SV40 T-ag is a 708–amino acid protein containing at least three independent functional domains: an N-terminal J domain (amino acids 1–130), a central origin binding domain (obd) (amino acids 131–260), and a C-terminal helicase domain (amino acids 266–625). In the case of SV40, a single virally encoded initiator, large T-antigen (T-ag), can bind the SV40 origin, assemble as a set of two hexameric rings, and cause local distortions (ie, melting) of the DNA. The T-ag obd recognizes the GAGGC-containing duplex DNA at the origin and also binds double-stranded DNA (dsDNA) and ssDNA in a non–sequence-specific manner. In this paper we describe two crystal structures of the SV40 large T-ag obd: one in complex with duplex DNA and one as a dimer in the absence of DNA.

The crystal structure of the SV40 T-ag obd (amino acids 131–260) with duplex DNA containing two high-affinity binding sites, P1 and P3, was refined to 2.4-Å resolution. Pentanucleotide binding site P2 has been altered to abrogate site-specific binding. The asymmetric unit contains two T-ag obd subunits and a DNA duplex 21 nucleotides long. The two T-ag obds are oriented head-to-head on approximately the same face of the DNA and make almost identical DNA interactions with their respective GAGGC sequences. The DNA positions the obds such that the residues within the B3 loop (amino acids 213–220) are facing each other in an antiparallel fashion, with Phe218 from one monomer and Thr217 from the other are close to one another but not quite contacting. Also in keeping with previous biochemical studies, each obd interacts with the DNA in the major groove primarily through the A1 (amino acids 147–159) and B2 (203–207) loops. Two residues within this motif, Asn153 and Arg154, make most of the base-specific interactions, with the pentanucleotide binding sites (P1 or P3). Residues adjacent or within the B2 loop (amino acids 202–204) interact primarily with the DNA phosphate backbone, with only Arg204 making sequence-specific interactions. The site-specific binding of the T-ag obd to DNA buries approximately 1,600 Å2 per GAGGC pentamer. The interaction of the two obds on P1 and P3 induces a 17-degree bend in the DNA.

>[2x]GSKVEDPKDFPSELLSFLSHAVFSNRTLACFAIYTTKEKAALLYKKIMEKYSVTFISRHNSYNHNILFFLTPHRHRVSAINNYAQKLCTFSFLICKGVNKEYLMYSALTRDPFSVIEESLPGGLKEHDFNPESS> MGGEIITLQAGQCGNHVGKFLWSQLAKEHAIGTDGLSQLPDSSTERDDDTKPFFRENCRNKFTPRAIMMDSEPSVIADVENTFRGFFDPRNTWVASDGASAGNSWANGYDIGTRNQDDILNKIDKEIDSTDNFEGFQLLHSVAGGTGSGLGSNLLEALCDRYPKKILTTYSVFPARSSEVVVQSYNTILALRRLIEDSDATVVFDNASLLNISGKVFRNPNIDLQHTNQLISTIISSVTNSIRFPSYMYSSMSSIYSTLIPSPELHFLSPSFTPFTSDYIHDDIAHKCHSSYDVMLDLLDPSNSLVSTAMNNPTYFNVYNTIIGNVEPRQISRAMTKLQQRIKFPSWSSSAMHVNIGRRSPYLPLQPNENEVS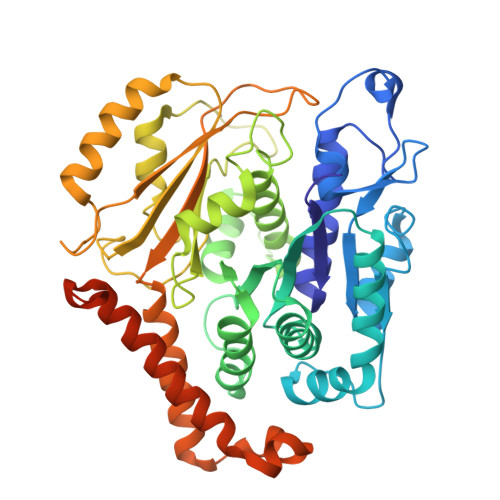GMMLSNMSTVVNVFENACNTFDKVFAKGAFLNNYNVGDLFQSMQNVQDEFAESREVVQSLMEDYVAAEQDSYLDDVLVDDENMVGELEEDLDADGDHKLV>[4x]MKQQEVRQRAFAMPLTSPAFPPGPYRFVNREYMIITYRTDPAAIEAVLPEPLQM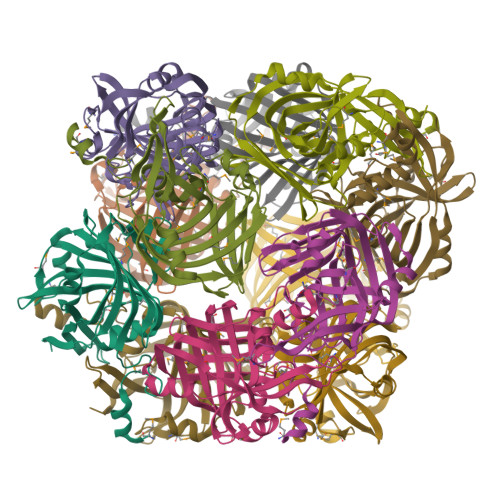AEPVVRYEFIRMPDSTGFGDYSESGQVIPVTFRGERGSYTLAMFLDDQPPLAGGRELWGFPKKAGKPRLEVHQDTLVGSLDFGPVRIATGTMGYKYEALDRSALLASLAEPNFLLKIIPHVDGSPRICELVRYHTTDVAIKGAWSAPGSLELHPHALAPVAALPVLEVLSARHFVCDLTLDLGTVVFDYLRQ> GTVQNPYADVK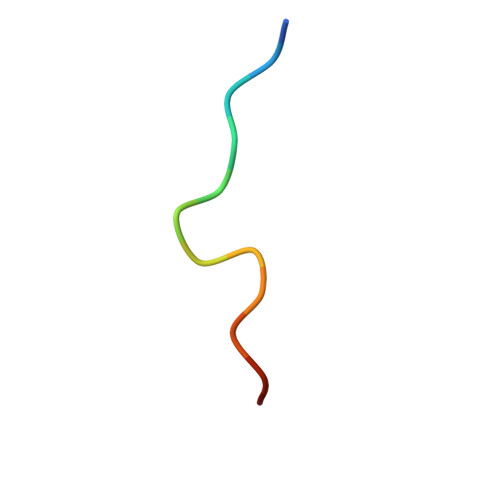TX>[2x]AELHNCVVVQFDGPMSFYVQMESDVPALEQMTDKLLDAEQDLPAFSDLKEGALCVAQFPEDEVFYRAQIRKVLDDG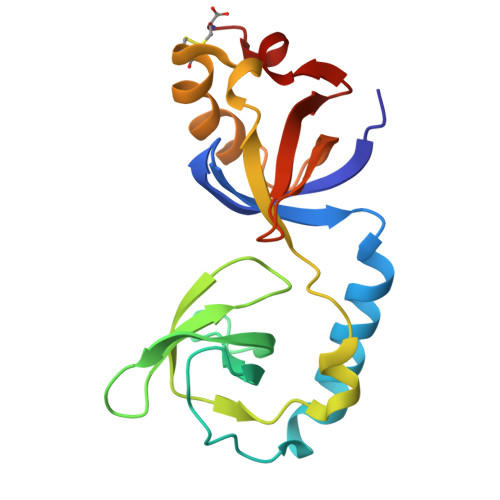KCEVHFIDFGNNAVTQQFRQLPEELAKPARYSRHCELDASTISKCDAALLQSFIDTRFSETFQVEILATKGTGTHVVRLFYQSKNISEKLQEC> GFPTELKPGTNQFLTTDDGVSAPILPNFHPTPCIHIPGEVRNLLELCQVETILEVNNVPTNATSLMERLRFPVSAQAGKGELCAVFRADPGRSGPWQSTLLGQLCGYYTQWSGSLEVTFMFTGSFMATGKMLIAYTPPGGPLPKDRATAMLGTHVIWDFGLQSSVTLV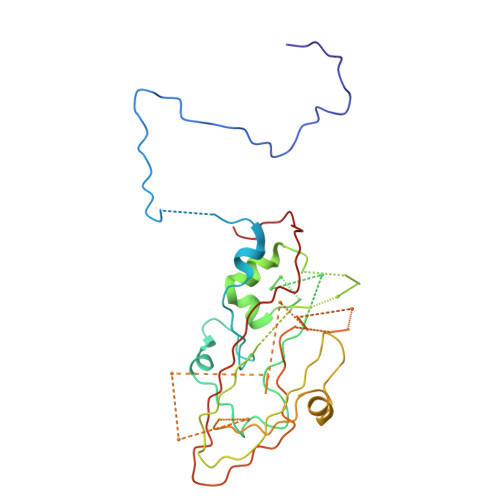IPTTGLVSIWYQTNYVVPIGAPNTAYIIALAAAQKNFTMQLCKDASDIL The contiguous latex includes an abundance of related proteins belonging to the pathogenesis-related (PR)10 family known collectively as major latex proteins (MLPs) and representing at least 35% of the total cellular protein content. Members of the pathogenesis-related (PR)10 family, also known as Bet v 1 or major latex proteins (MLPs), belong to the wider ‘StARkin’ lipid-transfer protein (LTP) classification with diverse physiological roles in plants, including sterol trafficking, lipid ‘sensor’ activity, and modulation of transcription factor function. Using a combination of sucrose density-gradient fractionation-coupled proteomics, differential scanning fluorimetry, isothermal titration calorimetry, and X-ray crystallography, we show that the major latex proteins are a family of alkaloid-binding proteins that display altered conformation in the presence of certain ligands. Seven antiparallel β-strands cradle the C-terminal α-helix with the alkaloid binding pocket located in a hydrophobic pocket between the central C-terminal α-helix and the β-sheet.

E76 hydrogen bonds directly with the isoquinoline moiety amine of papaverine and noscapine, and through a water molecule for (S)-tetrahydropapaverine. Alkaloid binding leads to the ordering of β2 completing the Bet v 1-fold. Alkaloid binding and subsequent ordering of the β2 strand causes C59 to be buried. Noscapine and papaverine showed the strongest binding affinity to all tested MLP/PR10 proteins in ANS-displacement assays with IC50 values from 4 to 126 μM and 42 to 493 μM, respectively. Notably, whereas ITC results suggested that a single MLP/PR10 protein binding-site could be occupied by two alkaloid ligand molecules, crystallography data showed that PR10 −10 bound only a single ligand. The size and flexibility of the binding pocket do not exclude the possibility that two alkaloids could potentially be accommodated. Crystallography and ITC results support a 1:1 and 2:1 binding ratio, respectively, which is insufficient to accommodate the direct binding of all accumulating BIA molecules. Our discovery of structural features unique to alkaloid-bound complexes, including S-S bonding, inform future studies regarding the nature and possible contributions of specific MLP/PR10 protein domains and quaternary structures.

> MAHHGVSGLVGKLVTQLEVNCDADIFYKIVKHHEEVPNVIPHFFTGVQVTKGDGLVSGCIKEWNYVLEGKAMTAVEETTHADETRTLTHHITEGDAMKDYKKFDVIVETNPKPNGHGSVVTYSIVYEKINEDSPAPFDYLKFFHQNIVDMSAHICSSA> GPLGSKEISEADKVIKATKETKETKKEVKRLKKEAKQRQQIPDHKKPQYASVDDTKTQALFDIYDTLNVNDKSFGDWFGNSALKDKTYLYAMDLLDYNNYLSIENPIIKTRAMGTYADLIIITGSLEQVNGYYNILKALNKRNAKFVLKINENMPYAQATFLRVPKRSDPNAHTLDKGASIDENKLFEQQKRAYFNYANDVICRPNDEVCSPLRD;> HHHHHHMDKLKDTPFMVQVKLPNYKDYLLDNKQVVLTFKLVHHSKKITLIGDANKILQYKNYFQANGARSDIDFYLQPTLNQKGVVMIASNYNDNPNSKEKP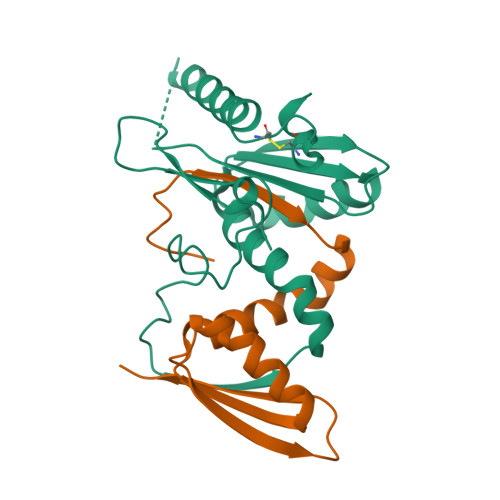QTFDVLQGSQPMLGANT(1S)-6-ethyl-N-{(1S)-1-[5-(2-ethyl-1-oxo-1,2-dihydroisoquinolin-6-yl)-1H-imidazol-2-yl]-7,7-dihydroxynonyl}-6-azaspiro[2.5]octane-1-carboxamide 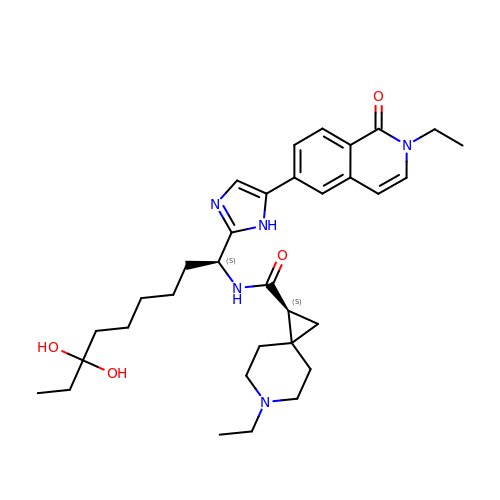| C33 H47 N5 O4 | UGJJVROKAWKMLZ-SXOMAYOGSA-N> GRLVGLELSNFKSYRGVTKVGFGESNFTSIIGPNGSGKSNMMDAISFVLGVRSNHLRSNILKDLIYRGVLSNPQSAYVKAFYQKGNKLVELMRIISRNGDTSYKIDGKTVSYKDYSIFLENENILIKAKNFLVFQGDVEQIAAQSPVELSRMFEEVSGSIQYKKEYEELKEKIEKLSKSAEEKKILNQFLKIKKKRKELFEKTFDYVSDHLDAIYRELTKNPNSNVELAGGNASLTIEDEDEPFNAGIKYHATPPLKRFKDMEYLSGGEKTVAALALLFAINSYQPSPFFVLDQVDAALDITNVQRIAAYIRRHRNPDLQFIVISLKNTMFEKSDALVGVYRQQQENSSKIITLDLSNYA;> GPYIKRVIIKGFKTYRNETIIDNFSPHQNVIIGSNGSGKSNFFAAIRFVLSDDYSNLKREERQGLIHQGSGGSVMSASVEIVFHDPDHSMILPSGVLSRGDDEVTIRRTVGLKKDDYQLNDRNVTKGDIVRMLETAGFSMNNPYNIVPQGKIVALTNAKDKERLQLLEDVVGAKSFEVKLKASLKKMEETEQKKIQINKEMGELNSKLSEMEQERKELEKYNELERNRKRAFENFKKFNERRKDLAERASELDESKDSIQDLIVKLKQQKVNAVDSTFQKVSENFEAVFERLVPRGTAKLIIHRYTGVSISVSFNSKQNEQLHVEQLSGGQKTVCAIALILAIQMVDPASFYLFDQIDAALDKQYRTAVATLLKELSKNAQFICTTFRTDMLQVADKFFRVKYENKISTVIEVNREEAIGFIR;> TLRTSGELLQGIVRVYSKQATFLLTDIKDTLTKISMLVIFTDVLKSITKREASRGFFDILSLATEGCIGLSQTEAFGNIKIDA;> MSYPGKDKNIPGRIIEALEDLPLSYLVPKDGLAALVNAPMRVSLPFDKTIFTSADDGRDVNINVLGTANSTTSSIKNEAEKERLVFKRPSNFTSSANSVDYVPTNFLEGLSPLAQSVLSTHKGLNDSINIEKKSEIVSRPEAKHKLESVTSNAGNLSFNDNSSNKKTKTSTGVTMTQANLAEQYLNDLKNILDIVGFDQNSAEIGNIEYWLQLPNKKFVLTTNCLTKLQMTIKNITDNPQLSNSIEITWLLRLLDVMVCNIKFSKSSLKMGLDDSMLRYIALLSTIVLFNIFLLGKNDSNLHRESYIMEPVNFLSDLIESLKILTIEYGSLKIEFDTFQEALELLPKYIRNGPFLDDNVTAKLVYIFSDLLMNNDIEATTNIQFQSFWDNVKRISSDILVSLFGSFDQQRGFIIEELLSHIEKLPTKRIQKKLRKVGNQNIYITDFTFTLMSMLENINCYSFCNQMKDIAPENIDLLKNEYKKQEEFLFNIVEHINDTILERFFKNPSALRYVIDNFVQDLLLLISSPQWPVTEKILSSLLKRLLSVYSPSMQVSANIETICLQLIGNIGSTIFDIKCSTRDHEDNNLIKMINYPETLPHFFKSFEECIAYNETIKCRRSATRFLWNLRLGTILILEEYTKDAKEQIITVDNELKKILEQIKDGGLGPELENREADFSTIKLDYFSILHAFELLNLYDPYLKLILSLLAKDKIKLRSTAIKCLSMLASKDKVILSNPMVKETIHRRLNDSSASVKDAILDLVSINSSYFEFYQQINNNYNDDSIMVRKHVLRINEKMYDETNDIVTKVYVIARILMKIEDEEDNIIDMARLILLNRWILKVHEVLDQPEKLKEISSSVLLVMSRVAIMNEKCSQLFDLFLNFYLLNKEAHSKEAYDKITHVLTILTDFLVQKIVELNSDDTNEKNSIVDKQNFLNLLAKFADSTVSFLTKDHITALYPYMVSDEKSDFHYYILQVFRCTFEKLANFKQKFLYDLETTLLSRLPKMNVREIDEAMPLIWSVATHRHDTARVAKACSSCLSHLHPYINKANNEEAAIVVDGKLQRLIYLSTGFARFCFPKPSNDKIAFLQEGETLYEHITKCLLVLSKDKITHVIRRVAVKNLTKLCGNHPKLFNSRHVLHLLDKEFQSDQLDIKLVILESLYDLFLLEERKSVRNTGVNSTLSSNSILKKKLLKTNRVEFANDGVCSALATRFLDNILQLCLLRDLKNSLVAIRLLKLILKFGYTNPSHSIPTVIALFASTSQYIRHVAYELLEDLFEKYETLVFSSLSRGVTKAIHYSIHTDEKYYYKHDHFLSLLEKLCGTGKKNGPKFFKVLKRIMQSYLDDITDLTSTNSSVQKSIFVLCTNISNITFVSQYDLVSLLKTIDLTTDRLKEVIMDEIGDNVSSLSVSEEKLSGIILIQLSLQDLGTYLLHLYGLRDDVLLLDIVEESELKNKQLPAKKPDISKFSAQLENIEQYSSNGKLLTYFRKHVKDT

Protein complexes containing SMC and kleisin subunits organise the spatial arrangement, or topology, of DNAs in most if not all living organisms. All contain a pair of rod-shaped SMC proteins with a dimerisation domain, known as the hinge, at one end and an ABC-like ATPase domain at the other, separated by a ~ 50 nm long anti-parallel intra-molecular coiled coil. Their association creates V-shaped dimers whose apical ATPase head domains are interconnected by a kleisin subunit (Scc1) whose N-terminal domain forms a three-helix bundle with the coiled coil emerging from Smc3's ATPase head, called its neck, and whose C-terminal winged helical domain binds to the base (or cap) of Smc1's ATPase head to complete the ring. Scc2 is essential for cohesin’s ATPase activity, for its loading onto chromosomes, for maintaining cohesin’s chromosomal association during G1, and for cohesin’s ability to extrude loops in vitro.

To elucidate how DNA actually associates with EQEQ cohesin trimers in the presence of ATP and Scc2, but lacking Scc3, namely under conditions in which DNAs are clearly entrapped within E-S and E-K but not S-K compartments, we used cryo-EM to solve the structure of EQEQ cohesin trimers (Smc1, Smc3 and Scc1) bound to ATP, linear DNA (40 bp), and Scc2C2 (residues 151–1493) to a resolution of 3.4 Å. First and foremost, E-S/E-K entrapment does indeed arise from the clamping of DNA between Scc2 and engaged heads in the manner revealed by both high and medium resolution cryo-EM structures. Scc2 holds DNA by way of a curved basic and polar surface located around the transition between its neck and head regions. The surface, which causes the DNA to bend slightly (~9°), is created by the spatial arrangement into a semicircle of a series of residues (e.g. S508, N557, K714, S753, S783, and K1324/25) from the ends of six α-helices and one loop (containing K427) that together engulf the phosphate backbone. This region includes all four positions mutated in Scc2-4E (S717E K721E K788E H789E), thus neatly explaining why the charge-reversing mutations lowered the binding affinity for DNA and inhibited entrapment of DNAs in vitro. Highly prominent is the binding of Scc2 to Smc1 through the docking of HEAT repeats 18–24 (residues 1127–1493) onto the F-loop (residues 1095–1118) on Smc1 head’s C-lobe and the coiled coils that emerge above. More conserved is a major contact mediated by salt bridges between a collection of highly conserved aspartate and glutamate residues located within two loops of Scc2 (819-EDEED-823 and 781-DD-782) and two key lysine residues (K112 K113) in Smc3. While Scc2 holds the upper half of the DNA’s backbone through a spiral of basic and polar residues, the engaged heads of Smc1 and Smc3 produce a 2-fold pseudo-symmetrical ABC ATPase heterodimer that binds DNA through two sites that are exactly two turns of the DNA apart and coincide with the major groove in the DNA.> GIVGVGIDLVSIPDFAEQVDQPGTVFAETF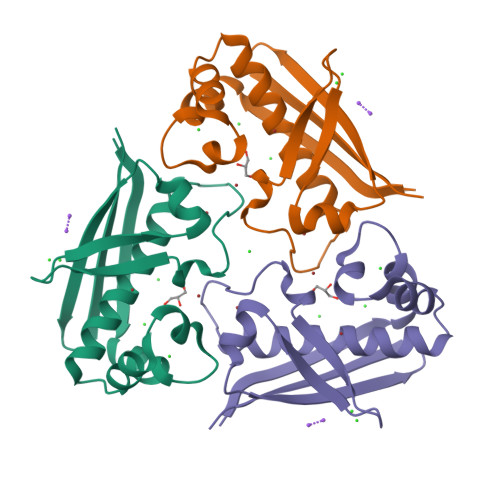TPGERRDASDKSSSAARHLAARWAAKEAVIKAWSGSRFAQRPVLPADIHRDIEVVTDMWGRPRVRLTGAIAEYLADVTIHVSLTHEGDTAAAVAILEAP> GSGGGGGSTQLNLRSLLVNPEGPTLMRLNSVQSSERPL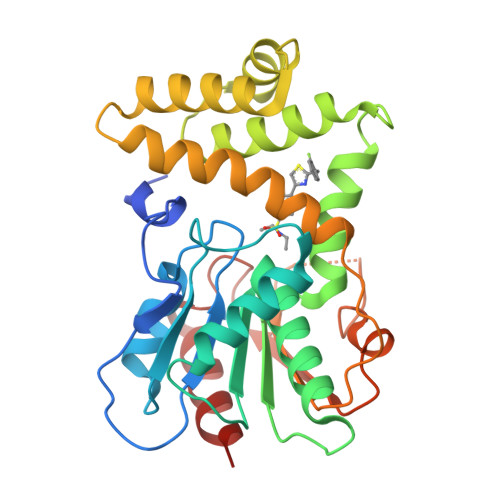FLVHPIEGSTTVFHSLASRLSIPTYGLQCTRAAPLDSIHSLAAYYIDCIRQVQPEGPYRVAGYSYGACVAFEMCSQLQAQQSPAPTHNSLFLFDGSPTYVLAYTQSYRAKLTPGCEAEAETEAICFFVQQFTDMEHNRVLEALLPLKGLEERVAAAVDLIIKSHQGLDRQELSFAARSFYYKLRAAEQYTPKAKYHGNVMLLRAKTGGAYGEDLGADYNLSQVCDGKVSVHVIEGDHRTLLEGSGLESIISIIHSSLAEH> SNAMIYEFVMTDPKIKYLKDYKPSNYLIDETHLIFELDESKTRVTANLYIVANRENRENNTLVLDGVELKLLSIKLNNKHLSPAEFAVNENQLIINNVPEKFVLQTVVEINPSANTSLEGLYKSGDVFSTQCEATGFRKITYYLDRPDVMAAFTVKIIADKKKYPIILSNGDKIDSGDISDNQHFAVWKDPFKKPCYLFALVAGDLASIKDTYITKSQRKVSLEIYAFKQDIDKCHYAMQAVKDSMKWDEDRFGLEYDLDTFMIVAVPDFNAGAMENKGLNIFNTKYIMASNKTATDKDFELVQSVVGHEYFHNWTGDRVTCRDWFQLSLKEGLTVFRDQEFTSDLNSRDVKRIDDVRIIRSAQFAEDASPMSHPIRPESYIEMNNFYTVTVYNKGAEIIRMIHTLLGEEGFQKGMKLYFERHDGQAVTCDDFVNAMADANNRDFSLFKRWYAQSGTPNIKVSENYDASSQTYSLTLEQTTLPTADQKEKQALHIPVKMGLINPEGKNIAEQVIELKEQKQTYTFENIAAKPVASLFRDFSAPVKVEHKRSEKDLLHIVKYDNNAFNRWDSLQQIATNIILNNADLNDEFLNAFKSILHDKDLDKALISNALLIPIESTIAEA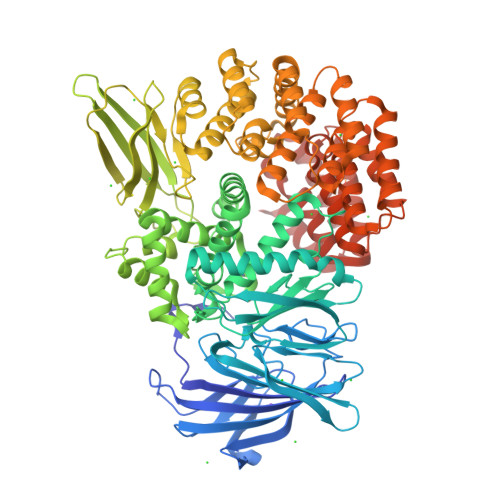MRVIMVDDIVLSRKNVVNQLADKLKDDWLAVYQQCNDNKPYSLSAEQIAKRKLKGVCLSYLMNASDQKVGTDLAQQLFDNADNMTDQQTAFTELLKSNDKQVRDNAINEFYNRWRHEDLVVNKWLLSQAQISHESALDIVKGLVNHPAYNPKNPNKVYSLIGGFGANFLQYHCKDGLGYAFMADTVLALDKFNHQVAARMARNLMSWKRYDSDRQAMMKNALEKIKASNPSKNVFEIVSKSLES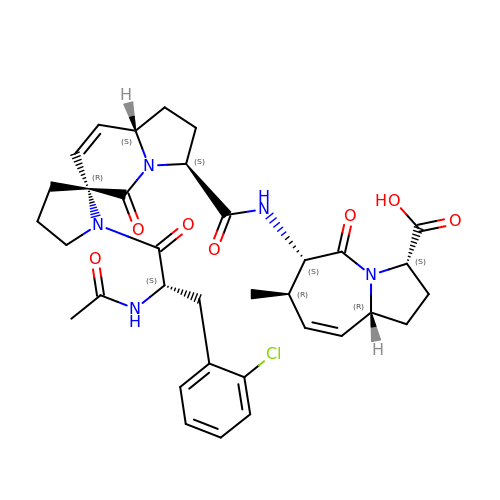(3~{S},6~{S},7~{R},9~{a}~{R})-6-[[(3~{S},6~{R},8~{a}~{S})-1'-[(2~{S})-2-acetamido-3-(2-chlorophenyl)propanoyl]-5-oxidanylidene-spiro[1,2,3,8~{a}-tetrahydroindolizine-6,2'-pyrrolidine]-3-yl]carbonylamino]-7-methyl-5-oxidanylidene-1,2,3,6,7,9~{a}-hexahydropyrrolo[1,2-a]azepine-3-carboxylic acid | C34 H40 Cl N5 O7 | WKURYOLGXNZIGX-WKYFTVTDSA-N>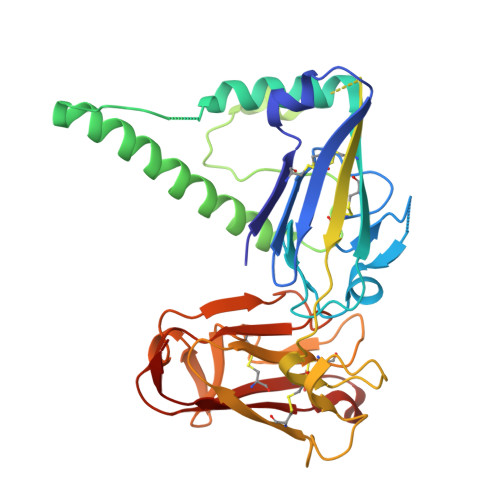 GASKSHKCDFTKEKYLLSGEKEVSCEIDANPSDDITFICPNKIDSLCFHTVNISKNINQNKSTMSIQDLLYGSVVYGNTLFISPYVRTNTPFYCFCNLDTVTIQKFLKINRFLKDDDELSEADVMKHLKGGNVSEAQADEYLNKALNRFKKMKDLSKFFNDQADNTTKLNLPKSLNIPNDILNYDVYNSSNNRNDIVVKDEVTNKQIISKRGIMSVFVRSNNNVIKGCDFGNNNKNYFSHPISVAGKVNNKVCKIQGKPGELVGFKCAFEENGKVEPPNCFDQVLHKNKVTDLKTLIPGYASYTNKHSSKYPYYLKIPHFVNEQYTIQCKCKSNNSQNEYTFELDIQPGES> MFVRSFCFLRKYGSKSKTPDLKTSFTKTTNFRKAEKISITTTDGEIVKGRGKIRRRTHSALKEAIGAMEHPAIWLWYPWRMNPEPPTPHMPQRRALKNVHGAVFNDLTPVQKKRQEQMLYGVNIPETRQMKFEEQHPLLAGALRKLEGQPKG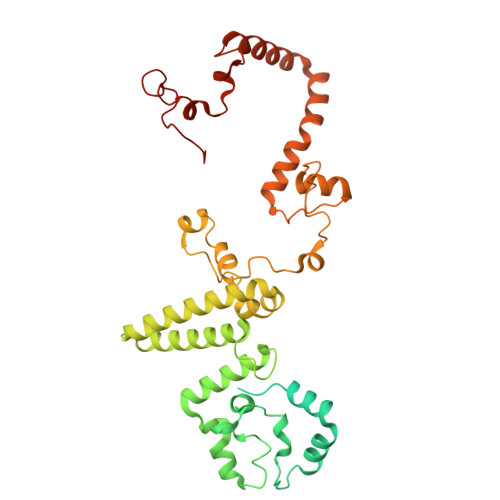FPFWYRKYPTRRHAYEYRFSIPVEMLDGYNDDVKKALSKGMMSIQEKQFAQEAMYMERYAEHDFDTTSPAVLAVKRALKCRVLRNHLLTNPHNNIIKTVLANTERKLNHALRRLRKVDFKKYWEIIRDHDVQDILQPPNLVTYRQGSYWKYDWNAGLAISTNLADVMDPRGLNGCVETGRSRSEVARDLGLSYTRPLHENEKKQLSHQAVYYERLAKFKMEQPEAARAMERERFVRKFSGMFVKMDIRSGAPDFPSTYRRLLGTKVVRWASKRHGPN In the barley β-d-glucan glucohydrolase, a glycoside hydrolase family 3 (GH3) enzyme, the Trp286/Trp434 clamp ensures β-d-glucosides binding, which is fundamental for substrate hydrolysis during plant growth and development. HvExoI folds into a two-domain structure consisting of an (α/β)8 barrel (domain 1) and an (α/β)6 sandwich (domain 2) with a 13 Å-deep active site pocket embracing the subsites −1 and +1, positioned at the interface between the two domains. HvExoI catalyses the hydrolytic removal of nonreducing glucose (Glc) moiety from a broad spectrum of poly- and oligomeric β-d-glucosides. The crucial role of substrate binding in HvExoI implies a pair of the aromatic Trp286 and Trp434 residues that form a clamp at the +1 subsite, which is positioned next to a pocket-shaped site at the −1 subsite, housing the Asp285 and Glu491 catalysts.

The G2SG-OMe thio-analogue bound weakly to native and WT recombinant HvExoI with the respective Ki of 2 ×10−3 M and 4 ×10−3 M, reflecting its ability to attach at the +1 and +2 subsites instead of the −1 and +1 subsites, which was most likely due to the rigidity of this thio-ligand. On the other hand, in W286F the electron density map of G2SG-OMe was defined at the −1 and +1 subsites, where this thio-ligand formed H-bonds with Asp95, Lys206, His207, Arg158, Tyr253, Asp285, Arg291, and Glu491, and stacking interactions with W286F and Trp434, whereas G2SG-OMe did not bind to W286A and W286Y.

> HHAADYVLYKDATKPVEDRVADLLGRMTLAEKIGQMTQIERLVATPDVLRDNFIGSLLSGGGSVPRKGATAKEWQDMVDGFQKACMSTRLGIPMIYGIDAVHGQNNVYGATIFPHNVGLGATRDPYLVKRIGEATALEVRATGIQYAFAPCIAVCRDPRWGRCYESYSEDRRIVQSMTELIPGLQGDVPKDFTSGMPFVAGKNKVAACAKHFVGDGGTVDGINENNTIINREGLMNIHMPAYKNAMDKGVSTVMISYSSWNGVKMHANQDLVTGYLKDTLKFKGFVISDFEGIDRITTPAGSDYSYSVKASILAGLDMIMVPNKYQQFISILTGHVNGGVIPMSRIDDAVTRILRVKFTMGLFENPYADPAMAEQLGKQEHRDLAREAARKSLVLLKNGKTSTDAPLLPLPKKAPKILVAGSHADNLGYQCGGWTIEWQGDTGRTTVGTTILEAVKAAVDPSTVVVFAENPDAEFVKSGGFSYAIVAVGEHPYTETKGDNLNLTIPEPGLSTVQAVCGGVRCATVLISGRPVVVQPLLAASDALVAAWLPGSEGQGVTDALFGDFGFTGRLPRTWFKSVDQLPMNVGDAHYDPLFRLGYGLTTNATKKY The fungal class D1 G-protein-coupled receptor (GPCR) Ste2 has a different arrangement of transmembrane helices compared with mammalian GPCRs and a distinct mode of coupling to the heterotrimeric G protein Gpa1–Ste2–Ste181. Ste2 is a homodimer that can couple to two G proteins simultaneously and its dimer interface is formed by the N terminus, extracellular loop 1 (ECL1) and transmembrane helices H1 and H7. Here we determined structures of Saccharomyces cerevisiae Ste2 in the absence of G protein in two different conformations bound to the native agonist α-factor, bound to an antagonist and without ligand. Activation of Ste2 requires both the removal of a blockage from the G protein coupling site (H7) and formation of the binding site primarily through the inward movement of H6.

We devised a method that we call pre-stabilization of a GPCR by weak association (PSGWAY) to purify Ste2–LF because of its inherent instability. The structures were determined by single particle cryo-EM to overall resolutions of 3.1 Å (ligand-free) and 2.7 Å (Ste2–Ant), with two separate structures of Ste2–Ag determined to resolutions of 3.5 Å. Mutation of F2045x28 and N2055x29 in this region abrogates both ligand binding and signalling, highlighting the importance of the conformational change. Agonist binding to the ligand-free inactive state of Ste2 causes reorientation of the extracellular end of H5 to facilitate ligand binding, an outward movement of the extracellular end of H6 and a shift of ECL3 (Ste2IL–Ag state), resulting in a contraction of the orthosteric binding site by an average of 27%. The dimer interfaces are smaller in ligand-free Ste2, Ste2–Ant and Ste2IL–Ag (2,166 Å2, 2,138 Å2 and 2,145 Å2, respectively) compared with Ste2AL–Ag and Ste2–Ag–G (2,727 Å2 and 2,519 Å2, respectively).

>MSDAAPSLSNLFYDPTYNPGQSTINYTSIYGNGSTITFDELQGLVNSTVTQAIMFGVRCGAAALTLIVMWMTSRSRKTPIFIINQVSLFLIILHSALYFKYLLSNYSSVTYALTGFPQFISRGDVHVYGATNIIQVLLVASIETSLVFQIKVIFTGDNFKRIGLMLTSISFTLGIATVTMYFVSAVKGMIVTYNDVSATQDKYFNASTILLASSINFMSFVLVVKLILAIRSRRFLGLKQFDSFHILLIMSCQSLLVPSIIFILAYSLKPNQGTDVLTTVATLLAVLSLPLSSMWATAANNASKTNTITSDFTTSTDRFYPGTLSSFQTDSINNDAKSSLRSRLYDLYPRRKETTSDKHSERTFVSETADDIEKNQFYQLPTPTSSKNTRIGPFADASYKEGEVEPVDMYTPDTAADEEARKFWTEDNNNL[2x]>[2x]GSHMVTDRDRLRPPLDERS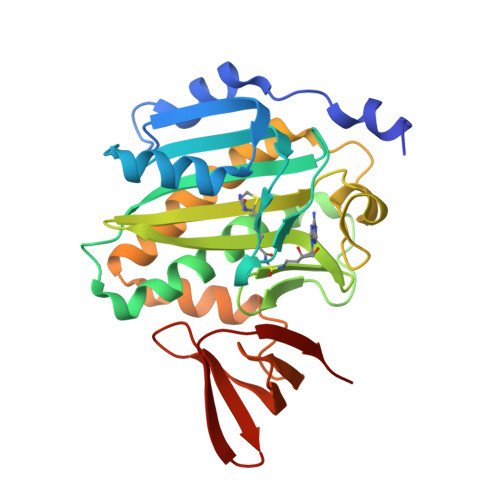LRDQLIGAGSGWRQLDVVAQTGSTNADLLARAASGADIDGVVLIAEHQTAGRGRHGRGWAATARAQIILSVGVRVVDVPVQAWGWLSLAAGLAVLDSVAPLIAVPPAETGLKWPNDVLARGGKLAGILAEVAQPFVVLGVGLNVTQAPEEVDPDATSLLDLGVAAPDRNRIASRLLRELEARIIQWRNANPQLAADYRARSLTIGSRVRVELPGGQDVVGIARDIDDQGRLCLDVGGRTVVVSAGDVVHLR> MRAHPGGGRCCPEQEEGESAAGGSGAGGDSAIEQGGQGSALAPSPVSGVRREGARGGGRGRGRWKQAGRGGGVCGRGRGRGRGRGRGRGRGRGRGRPPSGGSGLGGDGGGCGGGGSGGGGAPRREPVPFPSGSAGPGPRGPRATESGKRMDCPALPPGWKKEEVIRKSGLSAGKSDVYYFSPSGKKFRSKPQLARYLGNTVDLSSFDFRTGKMMPSKLQKNKQRLRNDPLNQNKG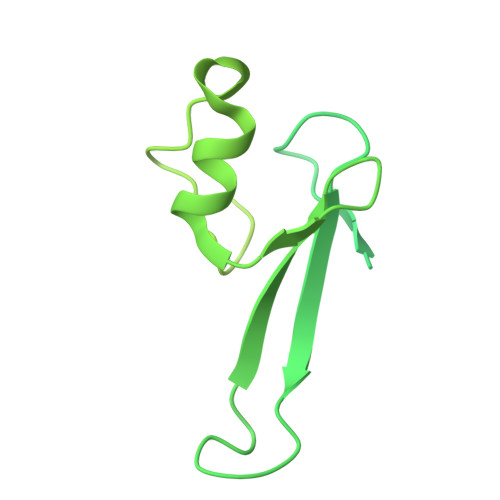KPDLNTTLPIRQTASIFKQPVTKVTNHPSNKVKSDPQRMNEQPRQLFWEKRLQGLSASDVTEQIIKTMELPKGLQGVGPGSNDETLLSAVASALHTSSAPITGQVSAAVEKNPAVWLNTSQPLCKAFIVTDEDIRKQEERVQQVRKKLEEALMADILSRAADTEEMDIEMDSGDEA> HDYELIAAPLDVELVPGFKTEAWAFGPSAPGTELRVRQGTWLRVRFINHLPVETTIHWHGIRLPLEMDGVPYVSQLPVKPGEFFDYKFRVPDAGSYWYHPHVSSSEELGRGLVGPLI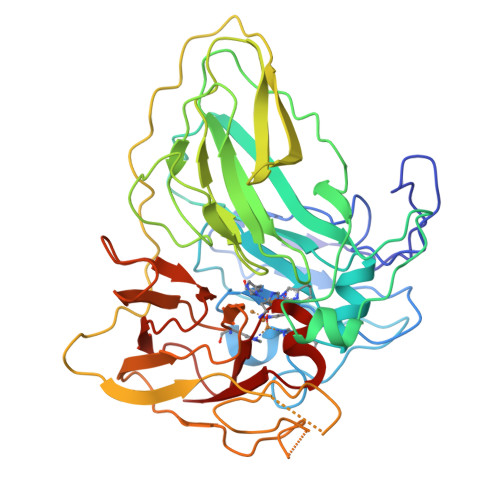VEEREPTGFLHERTLSLKTWHVDEQGAFMPFSVPREAARNGTAGRLITINGQAESVTELPAGQVVRVRLLNLDNTWTYRINLKGNCEAKVYALDGNPVTPRPLEDEYWLGPGMRICLAIRIPEAGEEISLRDGFVRLGTLRSVASSEAPGNWPKALPPNPIAEPDLEKAEKLNFNFEWAGKVSVDTDNGRPPSLWQINGQAWDITDKTCADRPIATLKKGKSYIFELKNMTQYQHPIHLHGMSFKVIASNRHKITEPWFTDTYLLGRNERAQVALVADNPGTWMFHCHVIDHMETGLMAAIAV> SIFKGSGVAIITPFTNTGVDFDKLSELIEWHIKSKTDAIIVCGTTGEATTMTETERKETIKFVIDKVNKRIPVIAGTGSN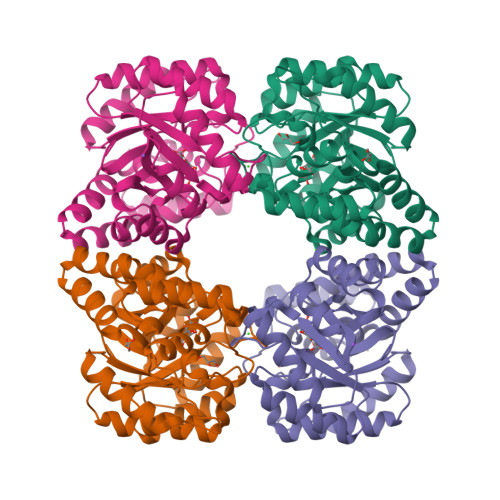NTAASIAMSKWAESIGVDGLLVITPYYNKTTQKGLVKHFKAVSDAVSTPIIIYNVPGRTGLNITPGTLKELCEDKNIVAVKEASGNISQIAQIKALCGDKLDIYSGNDDQIIPILALGGIGVISVLANVIPEDVHNMCELYLNGKVNEALKIQLDSLALTNALFIETNPIPVKTAMNLMNMKVGDLRLPLCEMNENNLEILKKELKAYNLM> GPLGSMSDENKSTPIVKASDITDKLKEDILTISKDALDKY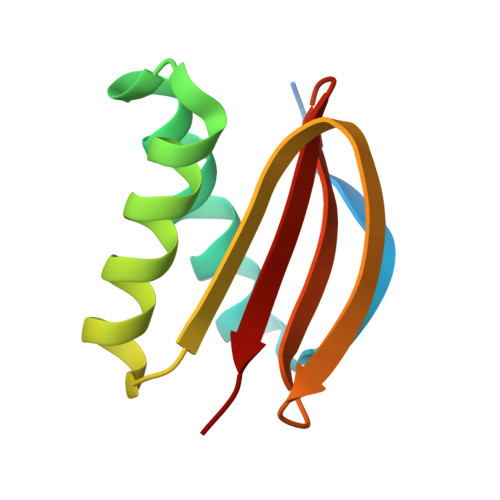QLERDIAGTVKKQLDVKYGNTWHVIVGKNFGSYVTHEKGHFVYFYIGPLAFLVFKTA> RDPTQFEERHLKFLQQLGKGNFGSVEMCRYDPLQDNTGEVVAVKKLQHSTEEHLRDFEREIEILKSLQHDNIVKYKGVCYSAGRRNLKLIMEYLPYGSLRDYLQKHKERIDHIKLLQYTSQICKGMEYLGTKRYIHRDLATRNILVENENRVKIGDFGLTKVLPQDKEYYKVKEPGESPIFWYAPESLTESKFSVASDVWSFGVVLYELFTYIEKSKSPPAEFMRMIGNDKQGQMIVFHLIELLKN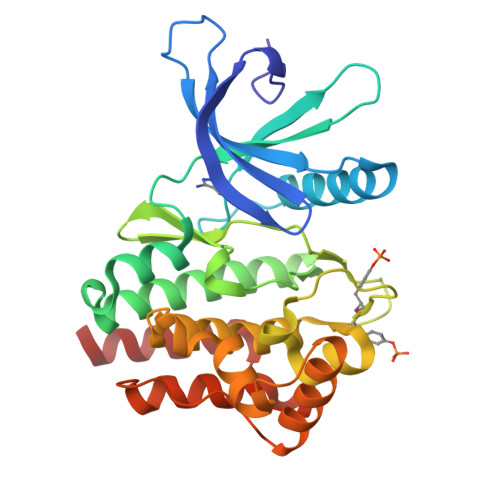NGRLPRPDGCPDEIYMIMTECWNNNVNQRPSFRDLALRVDQIRDNMA(5R)-5-{[10-(1,2,3,4-TETRAHYDROACRIDIN-9-YLAMINO)DECYL]AMINO}-5,6,7,8-TETRAHYDROQUINOLIN-2(1H)-ONE 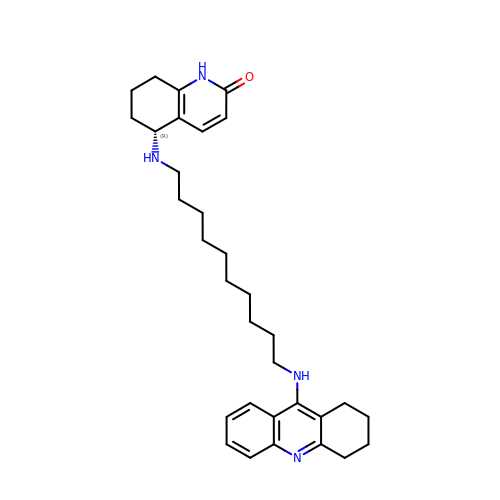| C32 H44 N4 O | ROTFGKJJMRTWBD-HHHXNRCGSA-N>AQKSVKISDDISITQLSDKVYTYVSLAEIEGWGMVPSNGMIVINNHQAALLDTPINDAQTEMLVNWVTDSL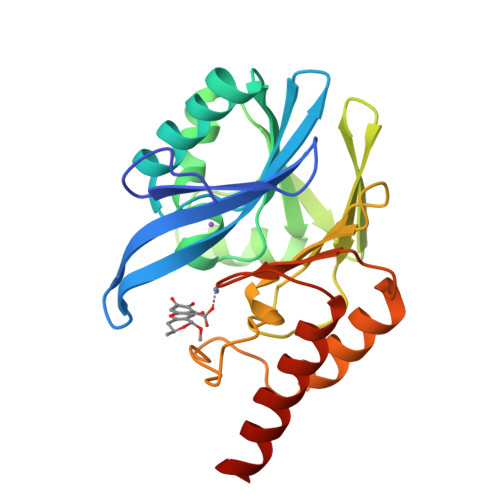HAKVTTFIPNHWHGDCIGGLGYLQRKGVQSYANQMTIDLAKEKGLPVPEHGFTDSLTVSLDGMPLQCYYLGGGHATDNIVVWLPTENILFGGCMLKDNQATSIGNISDADVTAWPKTLDKVKAKFPSARYVVPGHGDYGGTELIEHTKQIVNQYIESTSKP[2x]>PMVTIGPNGTEVSRISLSAINWAMTGPSITRKLLCEIFDRDTLAHHTLSGKPSPAFRDCARPSKQQLDPLKVADLVYLMTNSCDMTPREVRT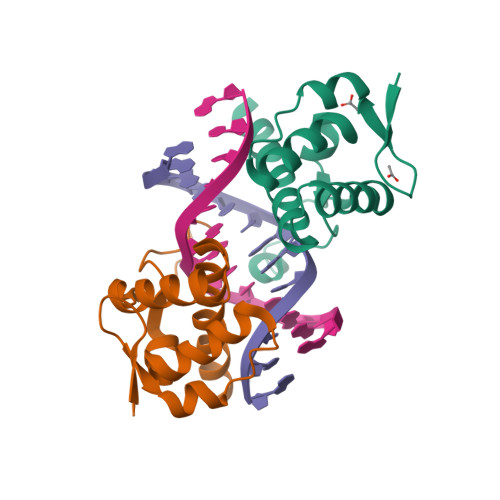AITTKCADENKMLRSRM[4x]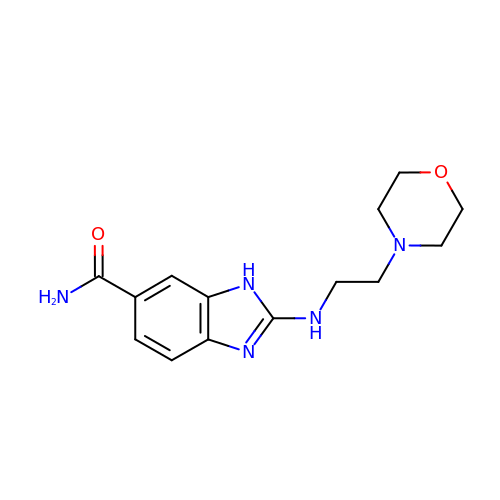2-{[2-(morpholin-4-yl)ethyl]amino}-1H-benzimidazole-6-carboxamide | C14 H19 N5 O2 | YAZZCCWYYDHQPD-UHFFFAOYSA-N3-(1-methylpyrrol-2-yl)benzoic acid | C12 H11 N O2 | 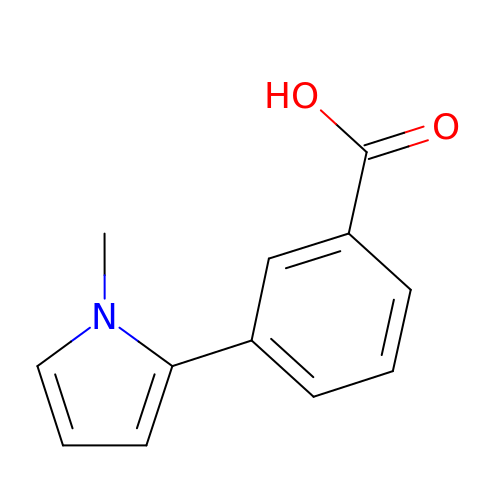UIRGFNLTEWMULM-UHFFFAOYSA-N> METDTLLLWVLLLWVPGSTGDLMVRSIQARLANKPKGTIKTIKGDDGEVVDCVDIYKQPAFDHPLLKNHTLQMQPSSYASKVGEYNKLEQPWHKNGECPKGSIPIRRQVITGLPVVKKQFPNLKFAPPSANTNHQYAVIAYFYGNASLQGANATINI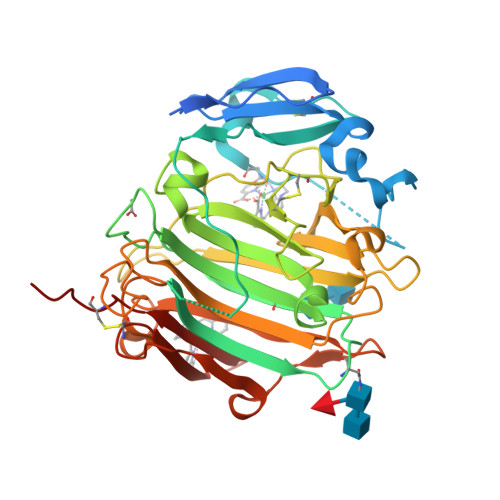WEPNLKNPNGDFSLTQIWISAGSGSSLNTIEAGWQVYPGRTGDSQPRFFIYWTADGYTSTGCYDLTCPGFVQTNNYYAIGMALQPSVYGGQQYELNESIQRDPATGNWWLYLWGTVVGYWPASIYNSITNGADTVEWGGEIYDSSGTGGFHTTTQMGSGHFPTEGYGKASYVRDLQCVDTYGNVISPTANSFQGIAPAPNCYNYQFQQGSSELYLFYGGPGCQAIAHHHHHH>GSSHHHHHHSSGRENLYFQGHMARPGMERWRDRLALVTGASGGIGAAVARALVQQGLKVVGCARTVGNIEELAAECKSAGYPGTLIPYRCDLSNEEDILSMFSAIRSQHSGVDICINNAGLARPDTLLSGSTSGWKDMFNVNVLALSICTREAYQSMKERNVDDGHIININSMSGHRVLPLSVTHFYSATKYAVTALTEGLRQELREAQTHIRATCISPGVV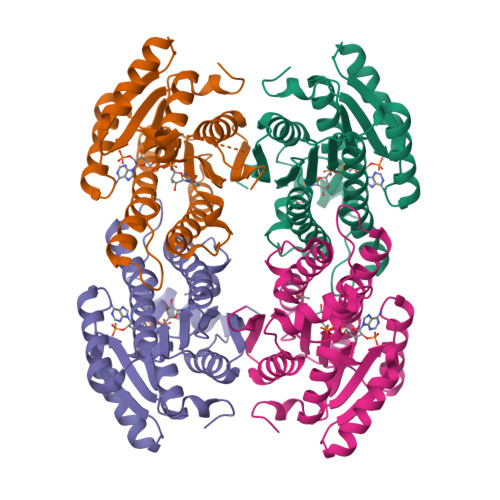ETQFAFKLHDKDPEKAAATYEQMKCLKPEDVAEAVIYVLSTPAHIQIGDIQMRPTGS[4x]>[40x]QAEILRA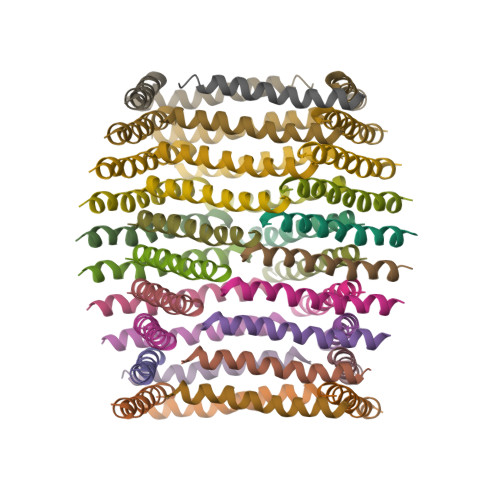YARILEADAKILEAHAEILKAQ>[2x]KT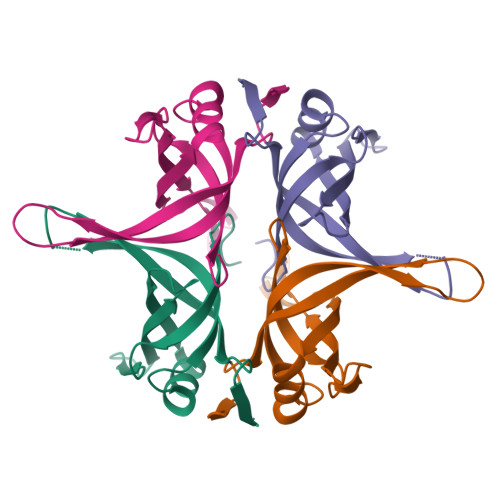MAGDTTITIVGNLTADPELRFTPSGAAVANFTVASTPRIYDRQTGEWKDGEALFLRCNIWREAAENVAESLTRGARVIVSGRLKQRSFETREGEKRTVIEVEVDEIGPSLRYATAKVNKASRSGGFGSGSRPAPAQTSSASGDDPWGSAPASGSFGGGDDEPPF> AEMEVQIVRNDPPLRYDTNLPVDLLHMVYAGRGATGSSGVVFGTWYRTIQDRTITDFPLTTRSADFRDGRMSKTFMTALVLSLQACGRLYVGQRHYSAFECAVLCLYLLYRNTHGAADDSDRAPVTFGDLLGRLPRYLACLAAVIGTEGGRPQYRYRDDKLPKTQFAAGGGRYEHGALASHIVIATLMHHGVLPAAPGDVPRDASTHVNPDGVAHHDDINRAAAAFLSRGHNLFLW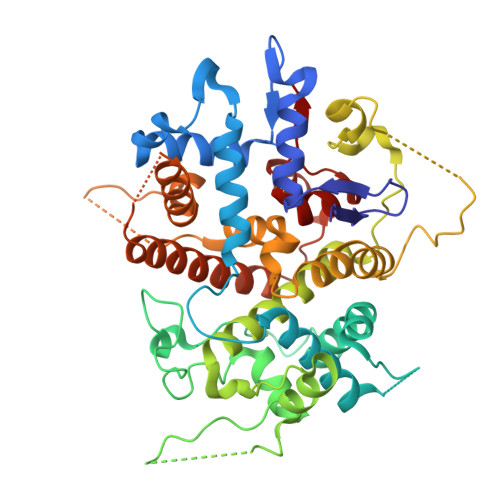EDQTLLRATANTITALGVIQRLLANGNVYADRLNNRLQLGMLIPGAVPSEAIARGASGSDSGAIKSGDNNLEALCANYVLPLYRADPAVELTQLFPGLAALCLDAQAGRPVGSTRRVVDMSSGARQAALVRLTALELINRTRTNPTPVGEVIHAHDALAIQYEQGLGLLAQQARIGLGSNTKRFSAFNVSSDYDMLYFLCLGFIPQYLSAV>[2x]AA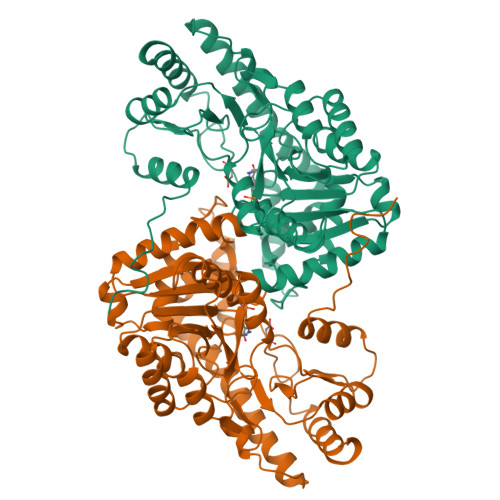SIFAAVPRAPPVAVFKLTADFREDGDSRKVNLGVGAYRTDEGQPWVLPVVRKVEQLIAGDGSLNHEYLPILGLPEFRANASRIALGDDSPAIAQKRVGSVQGLGGTGALRIGAEFLRRWYNGNNNTATPVYVSSPTWENHNSVFMDAGFKDIRTYRYWDAAKRGLDLQGLLDDMEKAPEFSIFILHACAHNPTGTDPTPDEWKQIAAVMKRRCLFPFFDSAYQGFASGSLDKDAWAVRYFVSEGFELFCAQSFSKNFGLYNERVGNLSVVGKDEDNVQRVLSQMEKIVRTTWSNPPSQGARIVATTLTSPQLFAEWKDNVKTMADRVLLMRSELRSRLESLGTPGTWNHITDQIGMFSFTGLNPKQVEYMIKEKHIYLMASGRINMCGLTTKNLDYVAKSIHEAVTKIQ> PIVGGHEG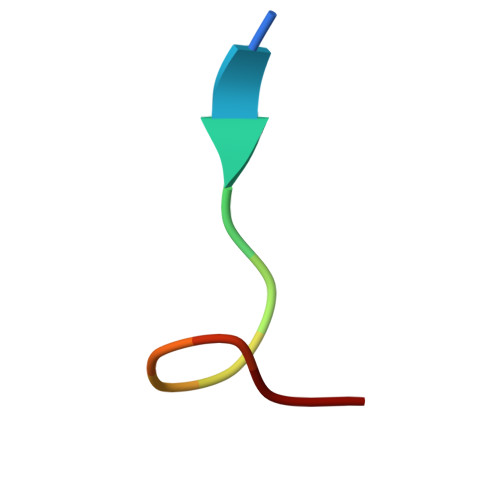AGV2'-DEOXYINOSINE 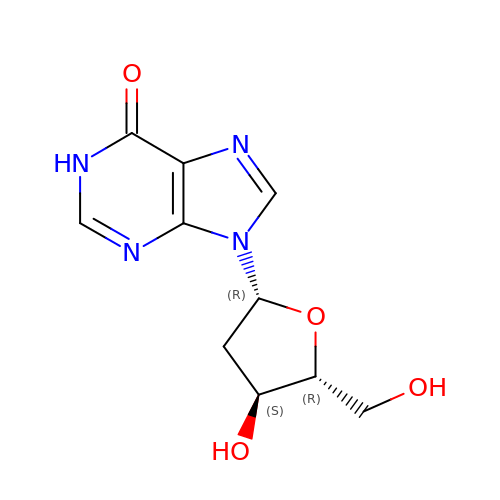| C10 H12 N4 O4 | VGONTNSXDCQUGY-RRKCRQDMSA-N>MASGSMHLRPIATPYPVKEWLQPKRYKAHLMGTTYVYDFPELFRQASSSQWKNFSADVKLTDDFFISNELIEDENGELTEVEREPGANAIGMVAFKITVKTPEYPRGRQFVVVANDITFKIGSFGPQEDEFFNKVTEYARKRGIPRIYLAANSGARIGMAEEIVPLFQVAWNDAANPDKGFQYLYLTSEGMETLKKFDKENSVLTERTVINGEERFVIKTIIGSEDGLGVECLRGSGLIAGATSRAYHDIFTITLVTCRSVGIGAYLVRLGQRAIQVEGQPIILTGASALNKVLGREVYTSNLQLGGTQIMYNNGVSHLTAVDDLAGVEKIVEWMSYVPAKRNMPVPILETKDTWDRPVDFTPTNDETYDVRWMIEGRETESGFEYGLFDKGSFFETLSGWAKGVVVGRARLGGIPLGVIGVETRTVENLIPADPANPNSAETLIQQAGQVWFPNSAFKTAQAINDFNNGEQLPMMILANWRGFSGGQRDMFNEVLKYGSFIVDALVDYKQPIIIYIPPTGELRGGSWVVVDPTINADQMEMYADVNARAGVLEPEGTVEIKFRREKLLDTMNRLDDKYRELRSQLSNKSLAPEVHQQISKQLADRERELLPIYG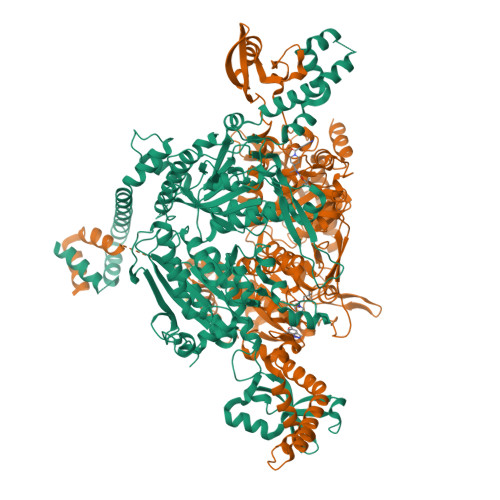QISLQFADLHDRSSRMVAKGVISKELEWTEARRFFFWRLRRRLNEEYLIKRLSHQVGEASRLEKIARIRSWYPASVDHEDDRQVATWIEENYKTLDDKLKGLKLESFAQDLAKKIRSDHDNAIDGLSEVIKMLSTDDKEKLLKTLKLEHHHHHH[2x]>TA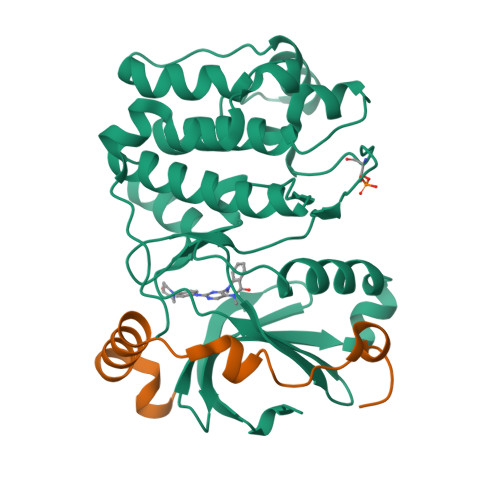LAEMPKRKFTIDDFDIGRPLGKGKFGNVYLAREKQNKFIMALKVLFKSQLEKEGVEHQLRREIEIQSHLRHPNILRMYNYFHDRKRIYLMLEFAPRGELYKELQKHGRFDEQRSATFMEELADALHYCHERKVIHRDIKPENLLMGYKGELKIADFGWSVHAPSLRRRTMCGTLDYLPPEMIEGKTHDEKVDLWCAGVLCYEFLVGMPPFDSPSHTETHRRIVNVDLKFPPFLSDGSKDLISKLLRYHPPQRLPLKGVMEHPWVKANSRRVLPPVYQSTQSK[2x];>[2x]PIPAWASGNLLTQAIRQQYYKPIDVDRMYGTIDSPKLEELFNKS Of particular interest in this context, is the role of the S-layer in disease. This paracrystalline protein array is the outermost layer of the C. difficile cell envelope, with similar structures found in many bacteria and virtually all archaea. In C. difficile, the main component of the S-layer is SlpA, which is post-translationally cleaved by a cell wall protein (CWP), Cwp84, into two functional S-layer proteins (SLPs), SLPL and SLPH. Assembly of the paracrystalline array relies on tiling of SLPH triangular prisms on the cell wall, interlocked by SLPL ridges facing the environment. Strikingly, the lattice is very compact compared to other studied S-layers, which have pores of between 30–100 Å compared with only ~10 Å in diameter in C. difficile.

An insertion of five-nucleotides was observed in a second variant, FM2.5slpA249insCTTAG (subsequently referred to as FM2.5varB; 249-253insCTTAG), resulting in the modification of 13 amino acids within the mature protein. Although crystals were obtained for all strains, only SlpAvarB crystals were of sufficient quality for X-ray diffraction data collection and structural determination by molecular replacement, using previous SlpA structures as models. The 13 altered residues in α2L in SlpAvarB result in disruption of the α-helix secondary structure and introduce disorder in the upstream loop that links the preceding β-strand (β3L) and α2L. However, the relative orientation of these domains in the SlpAvarB molecule is altered, with D1 and the interacting domains rotated towards the SLPH plane by ~30 °. In the SlpAvarB structure, disruption of α2L and reorientation of D1 and LID/HID relative to SLPH leads to changes in the interactions between neighbouring molecules and, consequently, a rearrangement of the S-layer array. Unlike in the previously determined structures, neighbouring D1 domains in the SlpAvarB structure are too far apart to mediate contacts (> 12 Å). A new interacting interface between HID from one molecule and CWB23 from a neighbouring molecule occludes these gaps and stabilises the S-layer lattice. The absence of density to model D2 in SlpAvarB further illustrates that this domain is dispensable for S-layer assembly, as previously reported. The presence of a more intricate network of interactions and more extensive interface areas between neighbouring molecules seen in the SlpAvarB structure, when compared to the R20291-related SlpARΔD2 structure, suggests a potentially less flexible paracrystalline array.

>[2x]AEDMSKVETGDQGYTVVQSKYKKAVEQLQKGLLDGSITEIKIFFEGTLASTIKVGAELSLVQKMQVNYCLHKVDNKLDNLGDGDYVDFLISSPAEGDKVTTSKLVALKNLTGGTSAIKVATSSIIGEVENAGTPGAKNTAPSSAAVMSMSDVFDTAFTDSTETAVKLTIKDAMKTKKFGLVDGTTYSTGLQFADGKTEKIVKLGDSDTINLAKELIITPASANDQAATIEFAKPTTQSGSPVITKLRILNAKEETIDIDASSSKTAQDLAKKYVFNKTDLNTLYRVLNGDEADTNRLVEEVSGKYQVVLYPEGKRVTTKS;>[2x]AAKASIADENSPVKLTLKSDKKKDLKDYVDDLRTYNNGYSNAIEVAGEDRIETAIALSQKYYNSDDENAIFRDSVDNVVLVGGNAIVDGLVASPLASEKKAPLLLTSKDKLDSSVKAEIKRVMNIKSTTGINTSKKVYLAGGVNSISKEVENELKDMGLKVTRLAGDDRYETSLKIADEVGLDNDKAFVVGGTGLADAMSIAPVASQLRNANGKMDLADGDATPIVVVDGKAKTINDDVKDFLDDSQVDIIGGENSVSKDVENAIDDATGKSPDRYSGDDRQATNAKVIKESSYYQDNLNNDKKVVNFFVAKDGSTKEDQLVDALAAAPVAANFGVTLNSDGKPVDKDGKVLTGSDNDKNKLVSPAPIVLATDSLSSDQSVSISKVLDKDNGENLVQVGKGIATSVINKLKDLLSM> ALVKEEIQAKEYLENLNKELAKRTNVETEAAWAYGSNITDENEKKKNEISAELAKFMKEVASDTTKFQWRSYQSEDLKRQFKALTKLGYAALPEDDYAELLDTLSAMESNFAKVKVCDYKDSTKCDLALDPEIEEVISKSRDHEELAYYWREFYDKAGTAVRSQFERYVELNTKAAKLNNFTSGAEAWLDEYEDDTFEQQLEDIFADIRPLYQQIHGYVRFRLRKHYGDAVVSETGPIPMHLLGNMWAQQWSEIADIVSPFPEKPLVDVSAEMEKQGYTPLKMFQMGDDFFTSMNLTKLPQDFWDKSIIEKPTDGRDLVCHASAWDFYLIDDVRIKQCTRVTQDQLFTVHHELGHIQYFLQYQHQPFVYRTGANPGFHEAVGDVLSLSVSTPKHLEKIGLLKDYVRDDEARINQLFLTALDKIVFLPFAFTMDKYRWSLFRGEVDKANWNCAFWKLRDEYSGIEPPVVRSEKDFDAPAKYHISADVEYLRYLVSFIIQFQFYKSACIKAGQYDPDNVELPLDNCDIYGSAAAGAAFHNMLSMGASKPWPDALEAFNGERIMSGKAIAEYFEPLRVWLEAENIKNNVHIGWTTSNKCVS;>WR[2x]

Angiotensin-I-converting enzyme (ACE, EC 3.4.15.1) is a promiscuous zinc metallopeptidase with a number of substrates, including the vasoregulatory peptides angiotensin I and bradykinin, the anti-fibrotic agent N-acetyl-SDKP, the neurotransmitter substance P, and amyloid-β peptide. Here, we present the use of the Drosophila melanogaster ACE homologue, AnCE (which, in particular, shares enzymatic properties with cACE), as a model to study the structural basis of ACE inhibition. The active site is located at the centre of this channel, marked by the location of the catalytic zinc ion, which is coordinated by His367, His371, and Glu395. The high-resolution crystal structures of AnCE in complex with the dipeptides VW, IW, YW, RW, and WR presented here reveal dual binding in both the non-prime (dipeptide-1) and prime (dipeptide-2) subsites of AnCE.

Due to ambiguity in the electron density maps, WR-1 was modelled in dual conformation in the non-prime subsites. In the first conformations, the arginine faces towards the S2 subsite, and the tryptophan sits within the S1 subsite, whereas in the second conformation, the dipeptide is flipped. In the first conformation, the arginine carboxyl group coordinates the zinc ion through a water-mediated interaction, whereas in the second conformation, the dipeptide distance from the zinc ion is too far for coordination. The observed Fo-Fc density makes a strong case for both conformations of WR-1. The WR-2 dipeptide was modelled in a single conformation; however, for this dipeptide, the side chain density is less continuous. As the WR dipeptide is the weakest binder out of all the dipeptides tested (Ki = 0.84 mM) in this report, the low occupancy would not be surprising. The arginine of the WR-2 sits within the S2′ pocket and forms H-bonds with Gln266, a hydrophobic contact with Phe441 and Phe511, and a salt bridge with Asp437. This binding also causes Gln266 to move (relative to the apo structure) in order to accommodate the arginine side chain within the subsite. The change in binding conformation of WR compared to the other dipeptides appears to be highly driven by the backbone interactions, in particular the carboxyl group, which occupies the polar pocket within the S2′ subsite. Out of all the dipeptides tested in this study, WR shows the highest Ki value for AnCE 840 µM (0.84 mM); this partially matches the findings of the study by Lunow et al., which showed that WR has a significantly higher specificity for nACE than cACE.> GVALGATRVIYPAGQKQEQLAVTNNDENSTYLIQSWVENADGVKDGRFIVTPPLFAMKGKKENTLRILDATNNQLPQDRESLFWMNVKAIPSMDKSKLTENTLQLAIISRIKLYYRPAKLALPPDQAAEKLRFRRS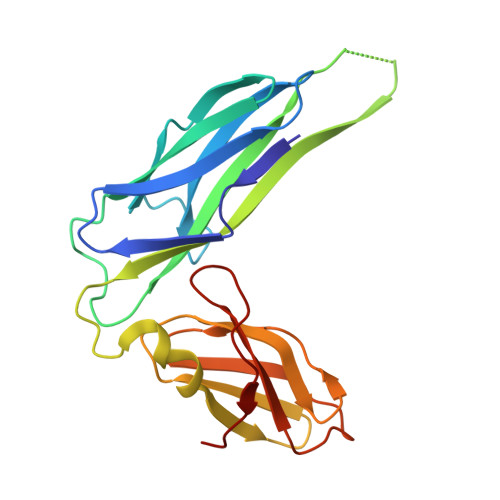ANSLTLINPTPYYLTVTELNAGTRVLENALVPPMGESTVKLPSDAGSNITYRTINDYGALTPKMTGVME> MQRRDFLKYSVALGVASALPLWSRAVFAAERPTLPIPDLLTTDARNRIQLTIGAGQSTFGGKTATTWGYNGNLLGPAVKLQRGKAVTVDIYNQLTEETTLHWHGLEVPGEVDGGPQGIIPPGGKRSVTLNVDQPAATCWFHPHQHGKTGRQVAMGLAGLVVIEDDEILKLMLPKQWGIDDVPVIVQDKKFSADGQIDYQLDVMTAAVGWFGDTLLTNGAIYPQHAAPRGWLRLRLLNGCNARSLNFATSDNRPLYVIASDGGLLPEPVKVSELPVLMGERFEVLVEVNDNKPFDLVTLPVSQMKMAIAPFDKPHPVMRIQPIAISASGALPDTLSSLPALPSLEGLTVRKLQLSMDPMLDMMGMQMLMEKYGDQAMAGMDHSQMMGHMGHGNMNHMNHGGKFDFHHANKINGQAFDMNKPMFAAAKGQYERWVISGVGDMMLHPFHIHGTQFRILSENGKPPAAHRAGWKDTVKVEGNVSEVLVKFNHDAPKEHAYMAHCHLLEHEDTGMMLGFTV

CueO, an MCOs from Escherichia coli (E. coli), together with CopA, a P-type ATPase, comprises a copper efflux (cue) system that resists copper stress under aerobic conditions. CueO can catalyze the oxidation of cuprous ion (Cu(I)) to the less toxic cupric ion (Cu(II)) in vivo. Previous analysis of the crystal structure of E. coli CueO has highlighted that it adopts a canonical architecture consisting of three similar cupredoxin-like domains linked by peptides. Very recently, we characterized the E. coli CueO G304K mutant (hereafter, G304K) from the metagenome of the sludge in a chemical plant, and found that catalytic efficiency of the mutant towards an organic substrate in the presence of excess Cu (II) was 2.7-folds higher than that of the wild-type enzyme.

In the present work, we report the crystal structure of G304K at a resolution of 1.49 Å. In the G304K crystal structure, although the T1 and T3 Cu atoms are fully occupied, T2 Cu atom is depleted. For G304K structure in native state, the occupancy for one of T3 Cu centre (Cu3) was as low as 20%, suggesting that it was almost depleted. When we examined the mutant protein crystal, we found no evidence of a Cu ion at the corresponding site in the structure. In the G304K mutant structure, the R-loop is not trapped in the mainly hydrophobic pocket, but sways away the core domain of the enzyme. Because of the bulky side chain and positive charge of the Lys residue in G304K mutant, the R-loop could be significantly repelled out of the hydrophobic pocket that is mainly formed by the MR helix. Noticeably, compared with the N-terminal part of the R-loop of the wild-type CueO (with or without excess Cu ions), the N-terminal part (residues 299–307) of the R-loop in the G304K mutant crystal structure significantly swayed in the absence of Cu ions. In contrast, the placement of the C-terminal part (residues 308–314) of the R-loop was almost not changed. Similar to most of the reported crystal structures of CueO, the loop (residues 370–398) near T1 Cu atom is disordered in the G304K structure, suggesting that it is flexible.>[2x]GPLGSAS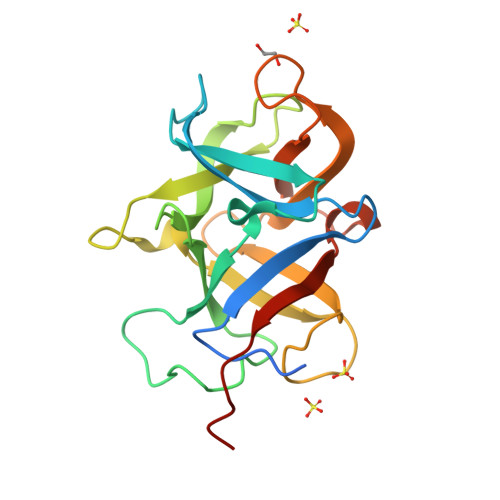AAASGKEGVEITYGSAIKLMHEKTKFRLHSHDVPYGSGSGQQSVTGFPGVVDSNSYWIVKPVPGTTEKQGDAVKSGATIRLQHMKTRKWLHSHLHASPISGNLEVSCFGDDTNSDTGDHWKLIIEGSGKTWKQDQRVRLQHIDTSGYLHSHDKKYQRIAGGQQEVCGIREKKADNIWLAAEGVYLPLNESSK> MSDLVNKKFPAGDYKFQYIAISQSDADSESCKMPQTVEWSKLISENKKVIITGAPAAFSPTCTVSHIPGYINYLDELVKEKEVDQVIVVTVDNPFANQAWAKSLGVKDTTHIKFASDPGCAFTKSIGFELAVGDGVYWSGRWAMVVE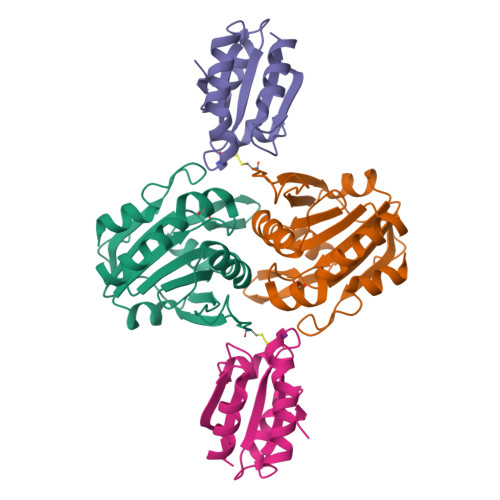NGIVTYAAKETNPGTDVTVSSVESVLAHL;> MGHHHHHHMVTQLKSASEYDSALASGDKLVVVDFFATWCGPSKMIAPMIEKFAEQYSDAAFYKLDVDEVSDVAQKAEVSSMPTLIFYKGGKEVTRVVGANPAAIKQAIASNV> GPLGSPLTASMLASAPPQEQKQMLGERLFPLIQAMHPTLAGKITGMLLEIDNSELLHMLESPESLRSKVDEAVAVLQAHQAKEAAQKA;> FVPNVHAAEFVPSFL

Cytoplasmic poly(A)-binding protein (PABP), also termed PABPC or PABPC1, is an essential protein that binds to and mediates the stimulatory effect of the poly(A) tail on translation initiation. Previous studies showed that MLLE is a peptide-binding domain that specifically recognizes a conserved PAM2 (for PABP-interacting motif 2) sequence. Unlike other PAM2-containing proteins, eRF3 possesses two overlapping PAM2 sequences (PAM2-N and PAM2-C), which each independently bind to the MLLE domain of PABPC1 with low micromolar affinity. Here, we determined two crystal structures of the MLLE domain of human PABPC1 in complex with the PAM2-N and PAM2-C peptides from human eRF3.

We obtained well-diffracting co-crystals with eRF3 residues 67–81 (PAM2-N) and 76–90 (PAM2-C). The C-terminal site (PAM2-C), in particular, lacks a leucine recognition element that is found in essentially all other PAM2 peptides. Overlay of the MLLE/PAM2-N and MLLE/PAM2-C structures reveals striking similarity of the bound conformations despite the highly divergent peptide sequences. The peptides adopt an extended conformation interrupted by a β-turn at residues Asn70-Val71-Asn72 in PAM2-N and at residues Asn79-Val80-His81 in PAM2-C. The most significant differences between the two peptide complexes occur at the N-terminus where PAM2-C lacks a highly conserved leucine residue. In its place, Phe76 bends back to partly occupy the space vacated by the missing leucine side chain. Thus eRF3 Phe76 plays two distinct roles in the complexes, alternately occupying the hydrophobic pocket between MLLE helices α2 and α3 in the PAM2-N complex and between helices α3 and α5 in the PAM2-C complex. Positions 1 and 2 are normally occupied by polar or charged residues, which do not participate in MLLE binding except in the MLLE/PAM2-C structure where phenylalanine in position 1 binds in combination with proline at position 3. Glutamic acid is preferred at position 9 and makes hydrogen bonds with amides of Gly579 and Lys580 in the PAM2-C structure via ordered water molecules. The simultaneous requirement for Phe76 for MLLE binding by both PAM2-N and PAM2-C explains the previous observations of a one-to-one stoichiometry of eRF3 binding to PABPC1 despite the existence of two PAM2 motifs.> MAVSATSQNTGDTVI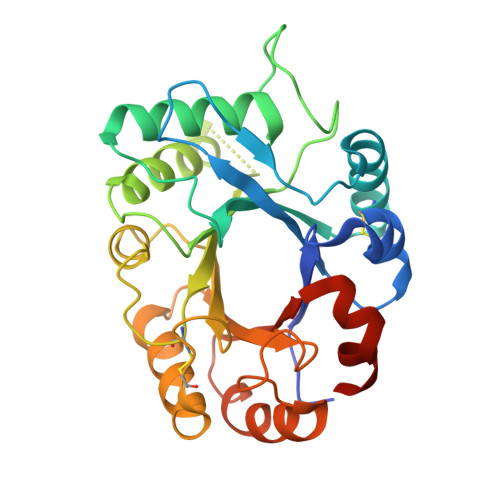IWGRNKDEGSLREACDAGRYTTVIISFLSAFGYIPGTYKLDISGHQVSAVGPDIKYCQSKGKLILLAIGGQGGEYSLPSSQAAVDLHDHLWYSYLGGRRNGVYRPFGDANVNGIDFFIDQGAREHYNELAKMLYDHNKDYRATVGVMVTATTRCGYPDHRLDEALATGLFHRIHVKMFSDGRCPAWSRRQSFEKWAKTYPQSRVLIGVVASPDVDKDAYMPPEALNNLLQFINKQPNFGGVMVWDRFYDKKTGFTAHLHHHHHH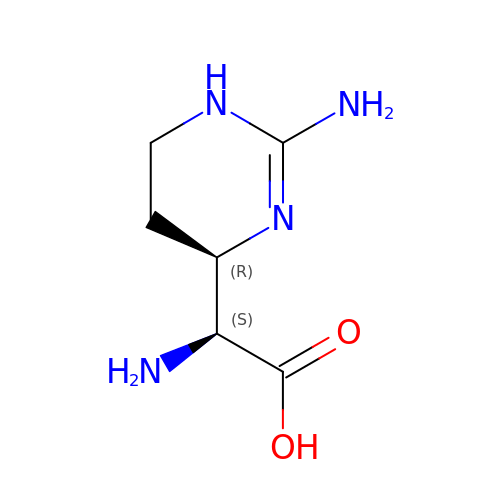(2S)-amino[(4R)-2-amino-1,4,5,6-tetrahydropyrimidin-4-yl]ethanoic acid | C6 H12 N4 O2 | XHNWDEHKMJLKGG-DMTCNVIQSA-N>MKPLSWSEAFGKGAGRIQASTIRELLKLTQRPGILSFAGGLPAPELFPKEEAAEAAARILREKGEVALQYSPTEGYAPLRAFVAEWIGVRPEEVLITTGSQQALDLVGKVFLDEGSPVLLEAPSYMGAIQAFRLQGPRFLTVPAGEEGPDLDALEEVLKRERPRFLYLIPSFQNPTGGLTPLPARKRLLQMVMERGLVVVEDDAYRELYFGEARLPSLFELAREAGYPGVIYLGSFSKVLSPGLRVAFAVAHPEALQKLVQAKQGADLHTPMLNQMLVHELLKEGFSER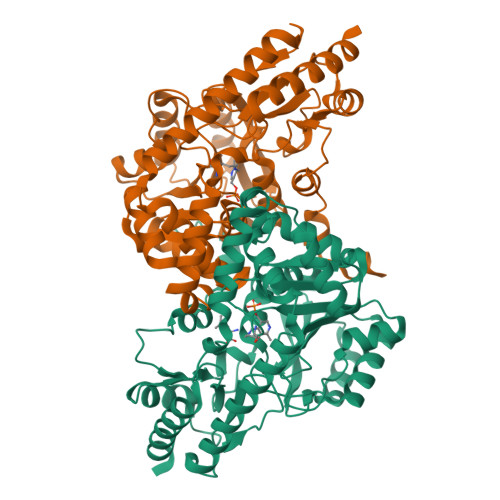LERVRRVYREKAQAMLHALDREVPKEVRYTRPKGGMFVWMELPKGLSAEGLFRRALEENVAFVPGGPFFANGGGENTLRLSYATLDREGIAEGVRRLGRALKGLLALV[6x]>CCG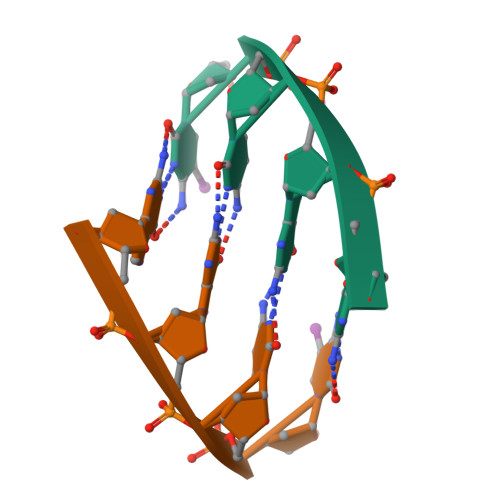G[2x]> QPQFNEDTLQQRLQALIESAGENWTYAIFWQISHDFDSSTGDNTVILGWGDGYYKGEEDKEKKKNNTNTAEQEHRKRVIRELNSLISGGIGVSDESNDEEVTDTEWFFLVSMTQSFVNGVGLPGESFLNSRVI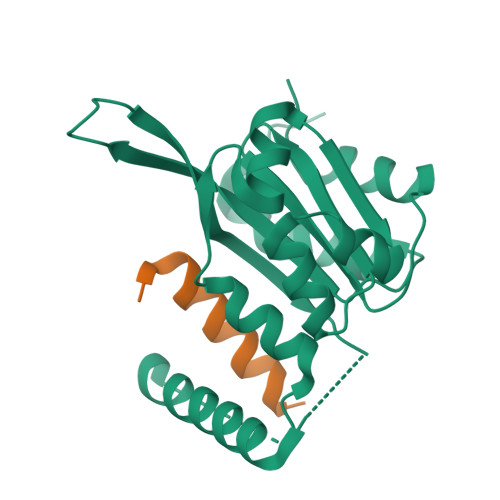WLSGSGALTGSGCERAGQGQIYGLKTMVCIATQNGVVELGSSEVISQSSDLMHKVNNLFNFN;> ELPIARRASLHRFLEKRKDRVT>MGIPADNLQSRAKASFDTRVAAAELALNRGVVPSFANGEELLXRNPDPDNTDPSFIASFTKGLPHDDNGAIIDPDDFLAFVRAINSGDEKEIADLTLGPARDPETGLPIWRSDLANSLELEVRGWENSSAGLTFDLEGPDAQSIAMPPAPVLTSPELVAEIAELYLMALGREIEFSEFDSPKNAEXIQFAIDQLNGLEWFNTPAKLGDPPAEIRRRRGEVTVGNLFRGILPGSEVGPYLSQYIIVGSKQIGSATVGNKTLVSPNAADEFDGEIAYGSITISQRVRIATPGRDFMTDLKVFLDVQDAADFRGFESYEPGARLIRTIRDLATWVHFDALYEAYLNACLILLANGVPFDPNLPFQQEDKLDNQDVFVNFGSAHVLSLVTEVATRALKAVRYQKFNIHRRLRPEATGGLISVNKIAAQKGESIFPEVDLAVEELGDILEKAEISNRKQNIADGDPDPDPSFLLPMAFAEGSPFHPSYGSGHAVVAGACVTILKAFFDSGIEIDQVFEVDKDEDKLVKSSFKGTLTVAGELNKLADNIAIGRNMAGVHYFSDQFESLLLGEQVAIGILEEQSLTYGENFFFNLP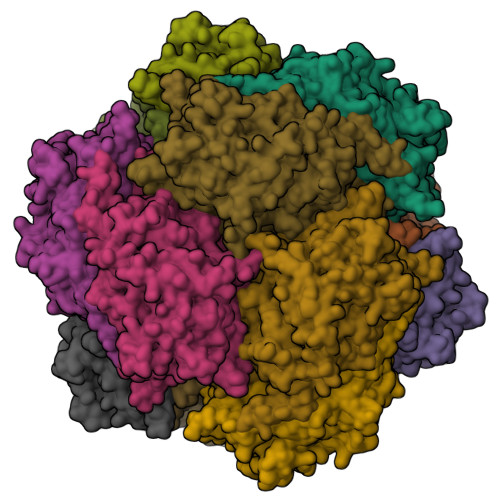KFDGTTIQI[4x]> MNYSYKRYWEPSTAEVIGLSLSVNTISAALTYPIEFVKVRSQIRTEGVGIRSKNLYMGINPNKVFREIHATGNGLRGFYQGFESHLIGRLSYLFIRNLTYKIIYDRTKPVKAHNDLSHREKGVIAGFAGGLAAFLTSPADLVNTRTIAEGGKPKEWR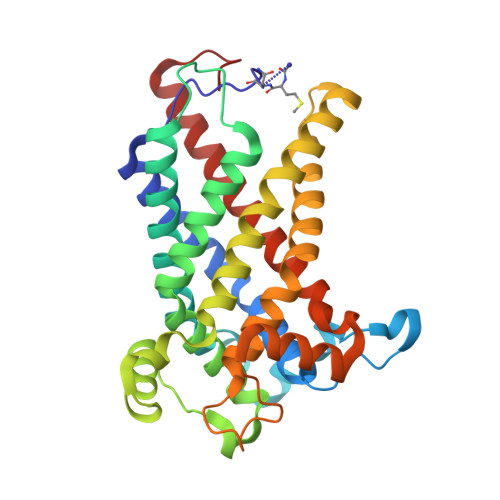WGYKGLMDGINKIAATEGGNAALFRGSYANVLRAVILNISLTGPFDYLNEKIWITFGDMTWNKYAALLWASFWGSVATLPFDNIRTRLYAQNADPTKNRLTYSGWADAAKKLIQHEGISGFYVGFYAFYIRTFLYAWTTVFITDKITSDWKRKAGLKEWQI>[2x]SADLALGKQTFEANCAACHAGGNNSVI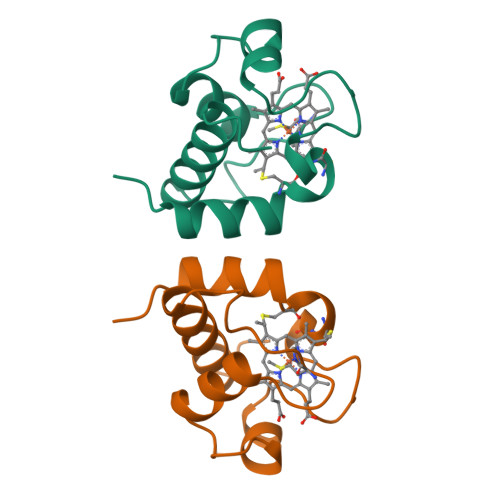PDHTLRKAAMEQFLQGGFNLEAITYQVENGKGAMPAWSGTLDDDEIAAVAAYVYDQASGDKW>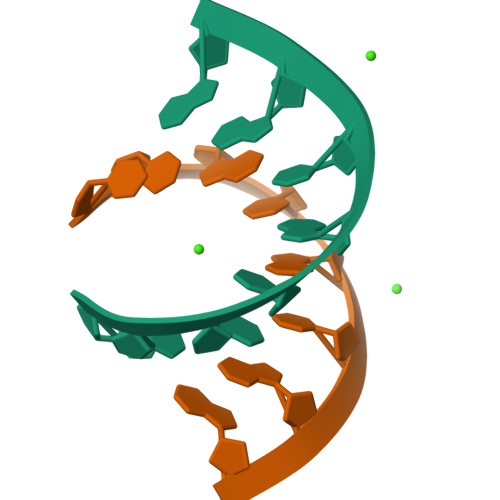[2x]UCGUACGA>[5x]MENRESAQRPHERLDAWRDSMELVEMIYRLTEVFPDQERYGLTAQLRRA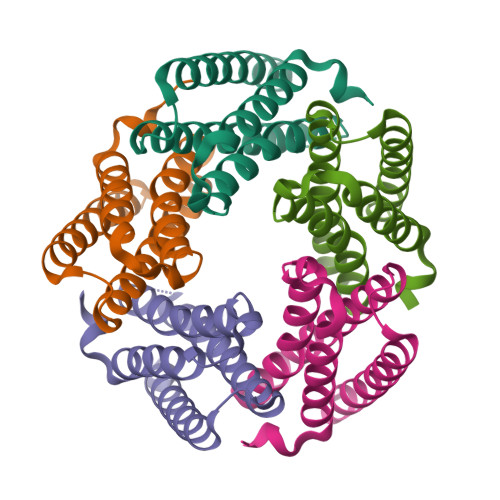AVSIPSNIAEGAARRSTPDYSRFLSIARGSLSELDTQVQIAARLGYSRSEDDQSVRRQVDLVFAKLTALMNALRRRGAA> KKEAEEVAAHVEQIAFIAKEQGNEEVAKLAKR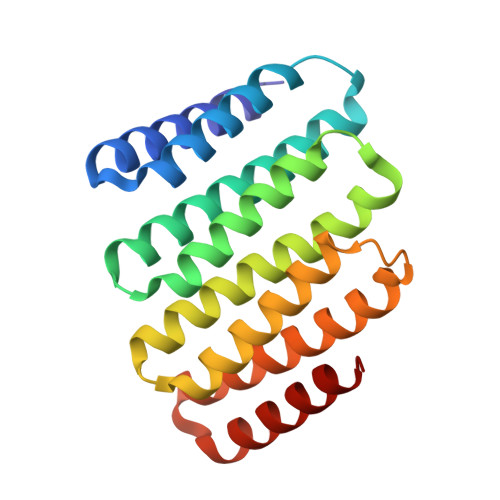LAETIKRLNEGTEEEVKRLLEAAEVAAHVLQIAFIAHEQGNEEVAKLALELAESILRLIEGTEEEVKRLLEAAEVAAHVLQIAFIAHEQGNEEVAKLALELAESILRLIEGTEEEVKELLERAEEAAHVLQHAFIATEQGNEEDAKEALRKAEEILRRNA(2S)-2-{4-[(2S)-4-[(6-aminopyridin-3-yl)sulfonyl]-2-(prop-1-yn-1-yl)piperazin-1-yl]phenyl}-3,3,3-trifluoropropane-1,2-diol | C21 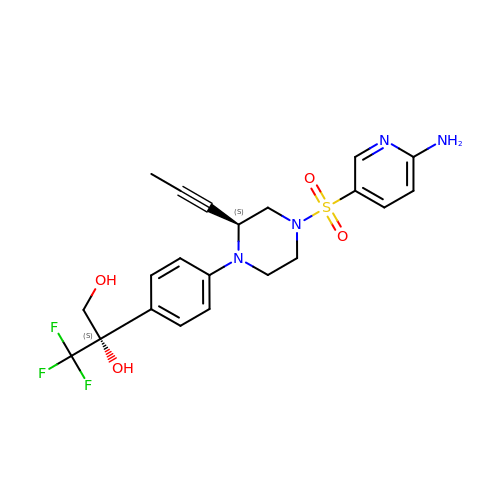H23 F3 N4 O4 S | HZYIALCWDCIMRP-FXAWDEMLSA-N> EEEEEDAGLVAEAEAVAAGWMLDFLCLSLCRAFRDGRSEDFRRTRNSAEA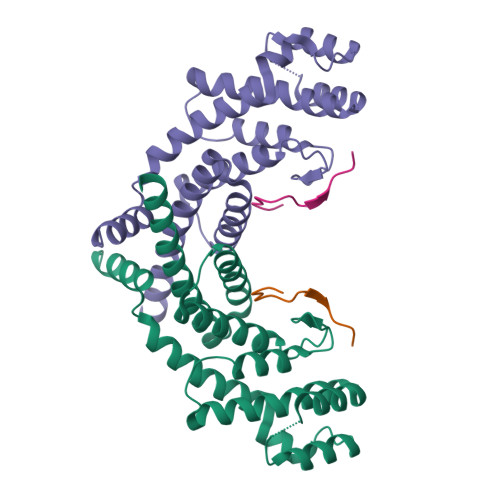IIHGLSSLTACQLRTIYICQFLTRIAAGKTLDAQFENDERITPLESALMIWGSIEKEHDKLHEEIQNLIKIQAIAVCMENGNFKEAEEVFERIFGDPNSHMPFKSKLLMIISQKDTFHSFFQHFSYNHMMEKIKSYVNYVLSEKSSTFLMKAAAKVVESKR;> SHFNLAPLGRRRVQSQWASTR>[3x]GPTPASYNLAVRRAAPAVVNVYNRGLNTNSHNQLEIRTLG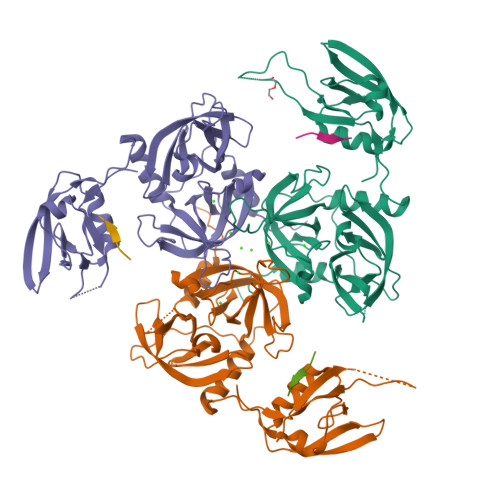SGVIMDQRGYIITNKHVINDADQIIVALQDGRVFEALLVGSDSLTDLAVLKINATGGLPTIPINARRVPHIGDVVLAIGNPYNLGQTITQGIISATGRIGLNPTGRQNFLQTDASINHGNSGGALVNSLGELMGINTLSFDKSNDGETPEGIGFAIPFQLATKIMDKLIRDGRVIRGYIGIGGREIAPLHAQGGGIDQLQGIVVNEVSPDGPAANAGIQVNDLIISVDNKPAISALETMDQVAEIRPGSVIPVVVMRDDKQLTLQVTIQEYPATN;>[3x]DNRLGLVYQF>[3x]MGSHHHHHHENLY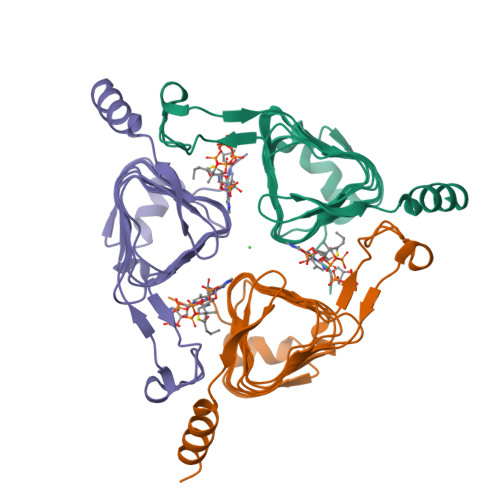FQGHMNSFYSQEELKKIGFLSVGKNVLISKKASIYNPGVISIGNNVRIDDFCILSGKVTIGSYSHIAAYTALYGGEVGIEMYDFANISSRTIVYAAIDDFSGNALMGPTIPNQYKNVKTGKVILKKHVIIGAHSIIFPNVVIGEGVAVGAMSMVKESLDDWYIYVGVPVRKIKARKRKIVELENEFLKSMNS Glycation, a non-enzymatic post-translational modification occurring on proteins, can be actively reversed via site-specific phosphorylation of the fructose-lysine moiety by FN3K kinase, to impact the cellular function of the target protein. Alternatively, the sugar moiety on glycated residues can be phosphorylated by a class of small-molecule kinases called fructosamine-3-kinases (FN3Ks), which are present in mammals, birds, and plants. Further characterization indicated that FN3K is responsible for protein deglycation by phosphorylating protein-associated fructosamines. Here, we determined a series of crystal structures of HsFN3K in the apo-state, and in complex with different nucleotide analogs together with a sugar substrate mimic to reveal the features important for its kinase activity and substrate recognition.

To understand how FN3K binds glycated substrates, we determined crystal structures of HsFN3K∆ in complex with ADP and a small molecule glycated substrate mimic, DMF. The protein fold is almost identical to the apo-HsFN3K∆ structure and exhibits unambiguous electron density for ADP and DMF in the nucleotide- and substrate-binding sites, respectively. A The crystal structure of HsFN3K in complex with ADP and the substrate DMF. Both protomers in the asymmetric unit contain ADP-DMF, while only protomer-1 shows a coordinated Mg2+ ion (green sphere). Several bulky amino acids (Pro71, Met88, His90, Met93, Phe39, and Tyr214) form a narrow pocket where the adenine base fits, stacked between the side chains of Phe39 and Met93. The two phosphates coordinate the Mg2+ ion in the catalytic site and are recognized by the highly conserved Lys41 residue. The positioning of Lys41 and the presence of a Mg2+ ion in the active site in HsFN3K support the placement of the nucleotide in a catalytically competent geometry, with both α and β phosphates directly coordinating the Mg2+ ion in an octahedral geometry along with Asp234 and Asn222 and two water molecules. The DMF sugar moiety binds in its linear tautomeric form in the substrate binding site, which is perfectly adapted to stabilize this active linear sugar geometry. His288 interacts directly with the morpholino group nitrogen via a H-bond. Asp217 establishes H-bonds with the sugar moiety with both O3’ and O4’ atoms. Upon ATP hydrolysis, the phosphate molecule is transferred onto the O3’ atom of the sugar moiety, and the crystal structure shows that the O3’ atom is positioned closest to the ADP in the catalytic center, directly interacting with one of the water molecules in the Mg2+ coordination sphere.

>[2x]AMEQLLRAELRTATLRAFGGPGAGCISEGRAYDTDAGPVFVKVNRRTQARQMFEGEVASLEALRSTGLVRVPRPMKVIDLPGGGAAFVMEHLKMKSLSSQASKLGEQMADLHLYNQKGSSYVDKFGFHTVTCCGFIPQVNEWQDDWPTFFARHRLQAQLDLIEKDYADREARELWSRLQVKIPDLFCGLEIVPALLHGDLWSGNVAEDDVGPIIYDPASFYGHSEFELAIALMFGGFPRSFFTAYHRKIPKAPGFDQRLLLYQLFNYLNHWNHFGREYRSPSLGTMRRLLK(2R)-1-(butanoyloxy)-3-{[(R)-hydroxy{[(1S,2S,3S,4S,5S,6R)-2,3,4,6-tetrahydroxy-5-(phosphonooxy)cyclohexyl]oxy}phosphoryl]oxy}propan-2-yl hexadecanoate | C29 H56 O16 P2 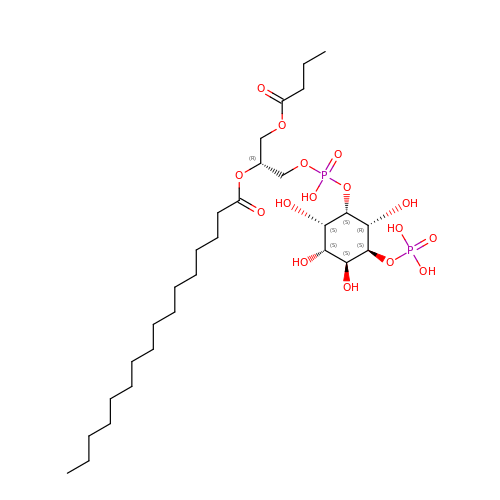| NJKPWDMBQIOYJP-IKLUZTLWSA-N2-[1'-(1~{H}-indazol-5-ylcarbonyl)-4-methyl-2-oxidanylidene-spiro[indole-3,4'-piperidine]-1-yl]-~{N}-[2,2,2-tris(fluoranyl)ethyl]ethanamide | C25 H24 F3 N5 O3 | 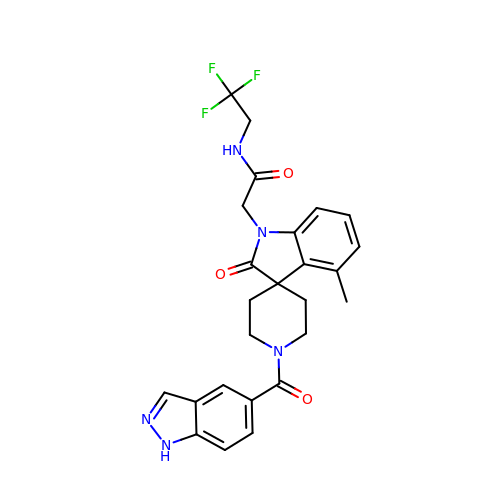OQTWZMQWXKMALD-UHFFFAOYSA-N TERT-BUTYL 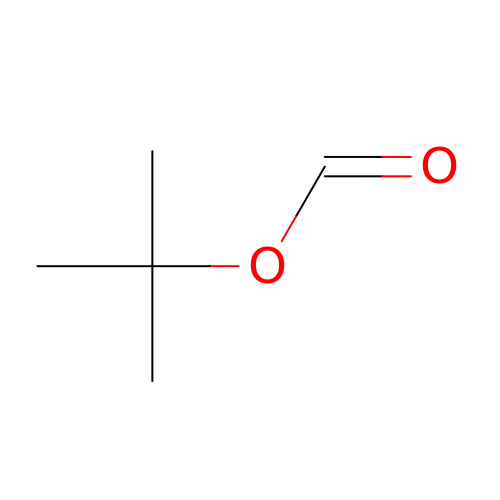FORMATE | C5 H10 O2 | RUPAXCPQAAOIPB-UHFFFAOYSA-N> MANRSHHNAGHRAMNALRKSGQKHSSESQLGSSEIGTTRHVY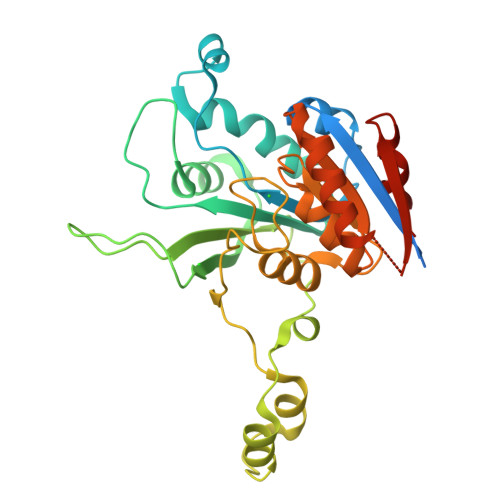DVCDCLDTLAKLPDDSVQLIICDPPYNIMPADWDDHMDYIGWAKRWLAEAERVLSPTGSIAIFGGLQYQGEAGSGDLISIISHMRQNSKMLLANLIIWNYPNGMSAQRFFANRHEEIAWFAKTKKYFFDLDAVREPYDEETKAAYMKDKRLNPESVEKGRNPTNVWRMSRLNGNSLERVGHPTQKPAAVIERLVRALSHPGSTVLDFFAGSGVTARVAIQEGRNSICTDAAPVFKEYYQKQLTFLQDDGLIDKARSYEIVEGAANFGAALQRGDVAS> MFVARSIAADHKDLIHDVSFDFHGRRMATCSSDQSVKVWDKSENGNWHCTASWKTHSGSVWRVTWAHPEFGQVLASCSFDRTAAVWEEIVGESNDKLRGQSHWVKRTTLVDSRTSVTDVKFAPKHMGLMLATCSADGVVRIYEAPDVMNLSQWSLQHEISCKLSCSCISWNPSSSR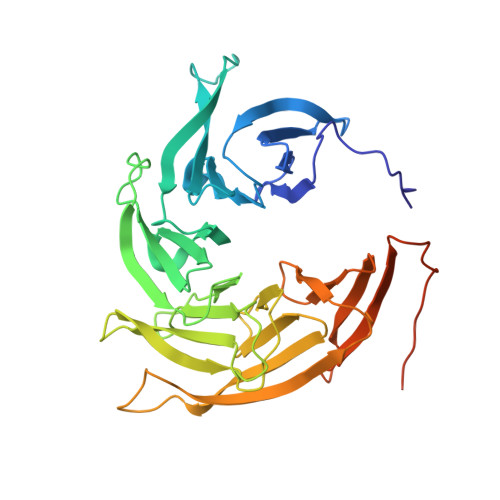AHSPMIAVGSDDSSPNIMGKVQIYEYNENTRKYAKAETLMSVSDPVHDIAFAPNLGRSFHILAVATKDVRIFTMKPLRKELSSSGGVTKFEIHTVAQFDNHNSQVWRVSWNITGTVLASSGDDGTVRLWKANYMDNWKCIGVLKGDGNPVGNSYQGFFGSSVGSAGQSLQNSVNGTPSSGRKHS>MAGKKVLIVYAHQEPKSFNGSLKNVAVDELSRQGCTVTVSDLYAMNFEPRATDKDITGTLSNPEVFNYGVETHEAYKQRSLASDITDEQKKVREADLVIFQFPLYWFSVPAILKGWMDRVLCQGFAFDIPGFYDSGLLQGKLALLSVTTGGTAEMYTKTGVNGDSRYFLWPLQHGTLHFCGFKVLAPQI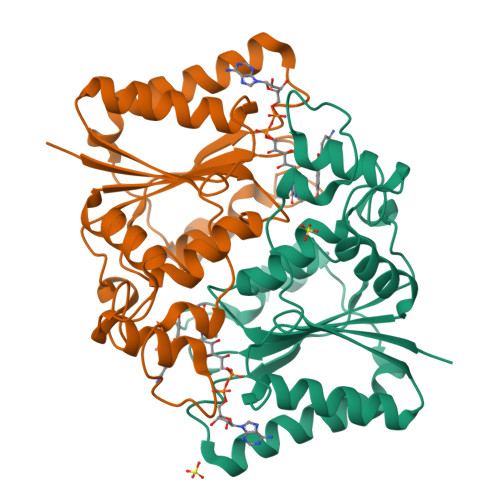SFAPEIASEEERKGMVAAWSQRLQTIWKEEPIPCTAHWHFGQ[2x]3-[3-(pyridin-3-yl)-1,2,4-oxadiazol-5-yl]benzonitrile | C14 H8 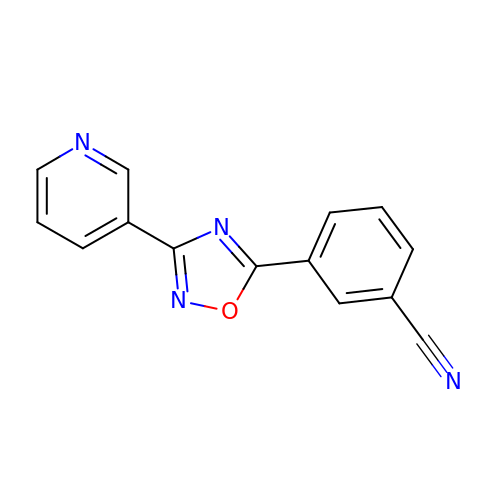N4 O | HGFXDSQLRSWUBO-UHFFFAOYSA-N4-METHYL-6-PROPYLPYRIDIN-2-AMINE | C9 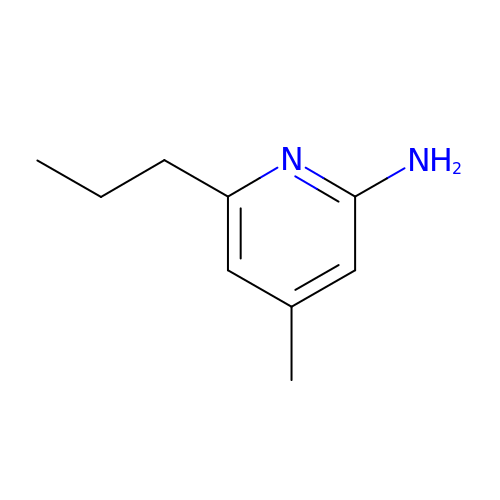H14 N2 | QGCCHDIBMYPTPX-UHFFFAOYSA-N>SLAKERQKKDNHNLIERRRRFNINDRIKELGTLIPKSNDPDMRWNKGTILKASVDYIRKLQREQQRA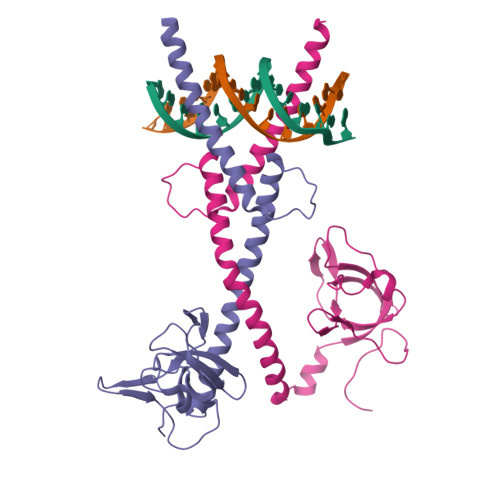KELENRQKKLEHACRHLLLRIQELGIEDFLKVDLRVAKVLSAERVEGSEKLLKLTLSLGDEERTVVAGIAKYYTPEELVGKKIVIVANLKPRKIFGIESQGMILAASDGENLSVIVPDRDVKEGAKLSAALE[2x]> QSPLLKEQIESIVIGKKATVGVAVWGPDDLEPLLINPFEKFPMQSVFKLHLAMLVLHQVDQGKLDLNQTVIVNRAKVLQNTWAPIMKAYQGDEFSVPVQQLLQYSVSHSDNVACDLLFELVGGPAALHDYIQSMGIKETAVVANEAQMHADDQVQYQNWTSMKGAAEILKKFEQKTQLSETSQALLWKWMVETT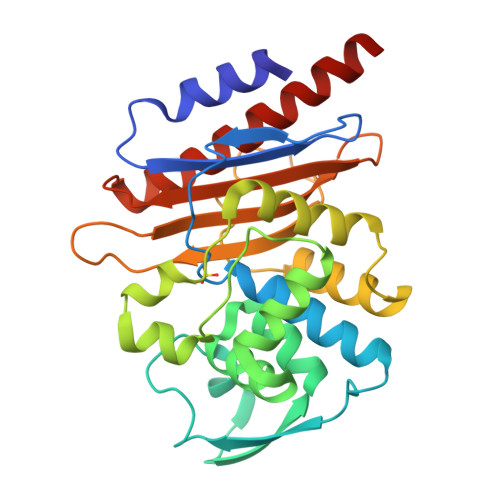TGPERLKGLLPAGTVVAHKTGTSQIKAGKTAATNDLGIILLPDGRPLLVAVFVKDSAESSRTNEAIIAQVAQTAYQFELKKLSALSPN> MKVVNLKQAILQAWKERWSDYQWAINMKKFFPKGATWDILNLAEALLEQAMIGPSPNPLILSYLKYAISSQMVSCSSVLTAISKFDDFSRDLCVQALLDIMDMFCDRLSCHGKAEECIGLCRALLSALHWLLRCTAASAERLQEGLEAGTPAPGEKQLALCLQCLEKTLSSTKNRALLHIAKLEEASSWTAIEHSLLKLGEILANLSNPQLRSQAERCGTLIRSIPSMLSVHSEQLHKTGFPTIHALILLEGTMNLTGEMQPLVEQLMMVKRMQHIPTPLFVLEIWKACFVGLIESPEGTQELKWTAFTYLKIPQVLVKLKKYFHGEKDFTEDVNCAFEFLLKLTPLLDKADQRCNCDCTNFLLQECNKQGLLSEVNFASLVGKRTADRDPQLKSSENANIQPNPGLILRAEPTVTNILKTMDADHSKSPEGLLGVLGHMLSGKSLDLLLAAAAATGKLKSFARKFINLNEFTTHGSGESTKTASVRALLFDISFLMLCHVAQTYGSEVILSESSSGEEVPFFETWMQTCMPEEGKILNPDHPCFRPDSTKVESLVALLNNSSEMKLVQMKWHEACLSISAAILEILNAWENGVLAFESIQKITDNIKGKVCSLAVCAVAWLVAHVRMLGLDEREKSLQMIRQLAGPLYSENTLQFYNERVVIMNSILEHMCADVLQQTATQIKFPSTGVDTMPYWNLLPPKRPIKEVLTDIFAKVLEKGWVDSRSIHILDTLLHMGGVYWFCNNLIKELLKETRKEHTLRAVQLLYSIFCLDMQQVTLVLLGHILPGLLTDSSKWHSLMDPPGTALAKLAVWCALSSYSSHKGQASSRQKKRHREDIEDYVSLFPVEDM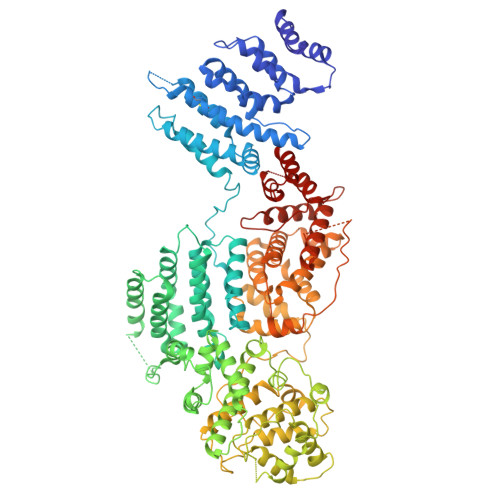QPSKLMRLLSSSDDDANILSSPTDRSMNSSLSASQLHTVNMRDPLNRVLANLFLLISSILGSRTAGPHTQFVQWFMEECVGCLEQDSRGSILQFMPFTTVSELVKVSAMSSPKVVLAITDLSLPLGRQVAAKAIAAL>[2x]GPELVMRRGEIWQVSLDAARGAEANNQRPAVVVSNDRANATATRLGRG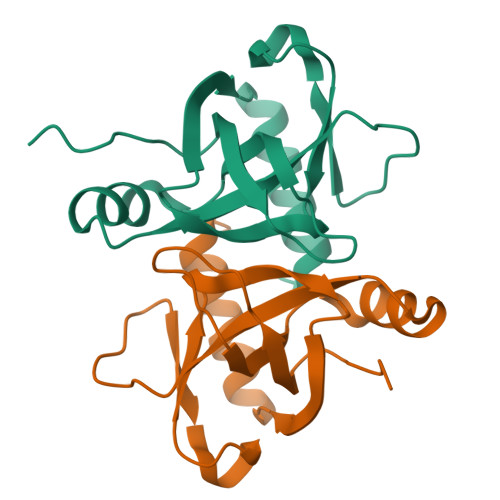VITVVPVTSNIAKVYPFQVLLSATTTGLQVDCKAQAEQIRSIATERLLRPIGRVSAAELAQLDEALKLHLDLWS>MGHHHHHHHHHHSSGHIEGRHMAPKRVVQLSLKMPTHAVCVVGVEAHVDIHSDVPKGANSFRVSGSSGVEVFMVYNRTRVKEPIGKARWPLDTDADMVVSVGTASKELKDFKVRVSYFGEQEDQALGRSVLYLTGVDISLEVDTGRTGKVKRSQGDKKTWRWGPEGYGAILLVNCDRDNHRSAEPDLTHSWLMSLADLQDMSPMLLSCNGPDKLFDSHKLVLNVPFSDSKRVRVFCARGGNSLSDYKQVLGPQCLSYEVERQPGEQEIKFYVEGLTFPDADFLGLVSLSVSLVDPGTLPEVTLFTDTVGFRMAPWIMTPNTQPPEELYVCRVMDTHGSNEKFLEDMSYLTLKANCKLTICPQVENRNDRWIQDEMEFGYIEAPHKSFPVVFDSPRNRGLKDFPYKRILGPDFGYVTREIPLPGPSSLDSFGNLDVSPPVTVGGTEYPLGRILIGSSFPKSGGRQMARAVRNFLKAQQVQAPVELYSDWLSVGHVDEFLTFVPTSDQKGFRLLLASPSACLKLFQEKKEEGYGEAAQFDGLKHQAKRSINEMLADRHLQRDNLHAQKCIDWNRNVLKRELGLAESDIVDIPQLFFLKNFYAEAFFPDMVNMVVLGKYLGIPKPYGPIINGRCCLEEKVQSLLEPLGLHCIFIDDYLSYHELQGEIHCGTNVRRKPFPFKWWN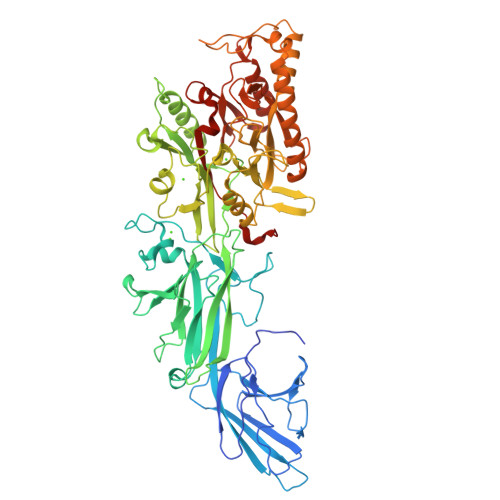MVP[2x]> MVEATAQETDRPRFSFSIAAREGKARTGTIEMKRGVIRTPAFMPVGTAATVKALKPETVRATGADIILGNTYHLMLRPGAE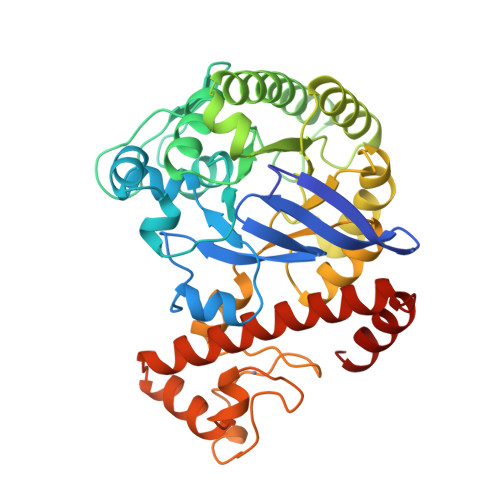RIAKLGGLHSFMGWDRPILTASGGYQVMSLSSLTKQSEEGVTFKSHLDGSRHMLSPERSIEIQHLLGSDIVMAFDECTPYPATPSRAASSMERSMRWAKRSRDAFDSRKEQAENAALFGIQQGSVFENLRQQSADALAEIGFDGYAVGGLAVGEGQDEMFRVLDFSVPMLPDDKPHYLMGVGKPDDIVGAVERGIDMFDCVLPTRSGRNGQAFTWDGPINIRNARFSEDLKPLDSECHCAVCQKWSRAYIHHLIRAGEILGAMLMTEHNIAFYQQLMQKIRDSISEGRFSQFAQDFRARYFARNS>HHHHHHSSGLVPRGSHMASMSKVGINGFGRIGRLVLRRLLEVKSNIDVVAINDLTSPKILAYLLKHDSNYGPFPWSVDFTEDSLIVDGKSIAVYAEKEAKNIPWKAKGAEIIVECTGFYTSAEKSQAHLDAGAKKVLISAPAGEM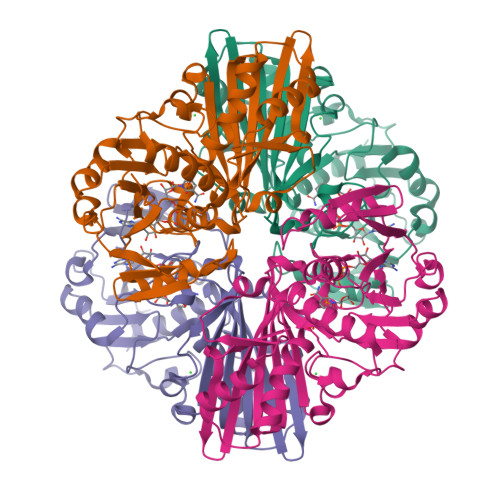KTIVYNVNDDTLDGNDTIVSVASSTTNCLAPMAKALHDSFGIEVGTMTTIHAYTGTQSLVDGPRGKDLRASRAAAENIIPHTTGAAKAIGLVIPELSGKLKGHAQRVPVKTGSVTELVSILGKKVTAEEVNNALKQATTNNESFGYTDEEIVSSDIIGSHFGSVFDATQTEITAVGDLQLVKTVAWYDNEYGFVTQLIRTLEKFAKL[4x]> DLIFCRKQAGVAIGRLCEKCDGKCVICDSYVRPCTLVRICDECNYGSYQGRCVICGGPGVSDAYYCKECTIQEK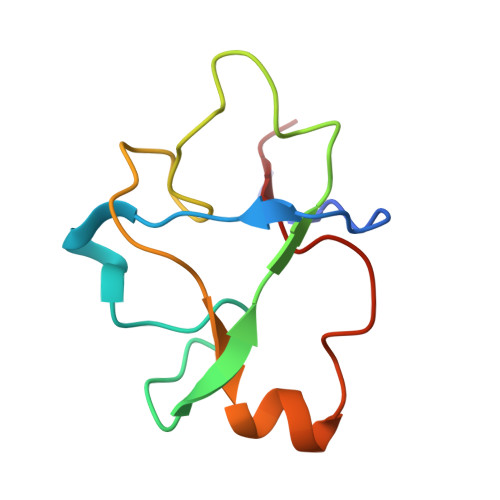DRDGCPKIVNL>SNAMRDNKYDILFEPVRIGPHIAKNRFYQVPHCNGGGYRDPSAAAAMRGIKSEGGWGVIFTEQTEMHHTSEITPFIELRLWEDKDIPGLRRMSDAMKVHGALAGIQLAYSGINGPNFYTKEVPLAPSALPIRTFTNDPVQARALDKQDIKNLRRWFVNAAKRSKIAGFDLICLYGAHGFGIFQHFLSRATNQRTDEYGGSLENRSRFAREVVEDIKEAVGDTTAITMRVSLDETIGELGFSNAEVREFVEMNANLPDLWDLAQGTWEDCSGPSRFKEEGAQEILVKGIRELSSKPVVGVGRFTSPDVMARMVRQGVLDFIGCARPSIADPFLPKKIEEGRIEDIRECIGCNICITGDMTMSISRCTQNPTFMEEWRKGWHPERMNAKGDSNTVLVVGAGPAGLEATRALSLRGYDVTLAEATTTLGGRVARERLLPGLSAWGRVVDYRQYQISQRTNVETYFDSRLTAEDVLGFGFEHVAIATGSHWRRDGVARQHVVPMPIDPSMTVWTPDDIMAKVHPENLSGKTVVVYDDDHYYMGGVMAEVMAKAGAKVILVTSSAYVSDWTRNTL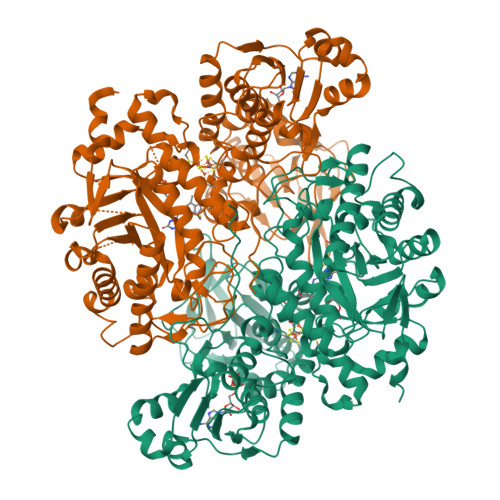EQGAIHVRLDDLGVDIRLNRGVTAIRAGEVETNCVYTGKRSAIGCDAVLMVASRTSEDQLFNDLIARQGDWPDAGIKSVKIIGDAAAPAPIAWATYAGHRYARELDTPDIGDDLPFRREVTQLEPA[2x]3-azanyl-2-[3-[2-[2-[2-[2-[2-[2-[2-[2-[2-[2-[2-[2-[2-[2-[2-[2-[2-[[3-azanyl-1-[[2-[[3-methyl-6-[4-methyl-3-(methylsulfonyl-$l^{2}-azanyl)cyclohexa-1,3,5-trien-1-yl]-[1,2,4]triazolo[4,3-b]pyridazin-8-yl]-$l^{2}-azanyl]-2-oxidanylidene-ethyl]amino]-1-oxidanylidene-propan-2-yl]amino]-2-oxidanylidene-ethoxy]ethoxy]ethoxy]ethoxy]ethoxy]ethoxy]ethoxy]ethoxy]ethoxy]ethoxy]ethoxy]ethoxy]ethoxy]ethoxy]ethoxy]ethoxy]ethoxy]propanoylamino]-~{N}-[3-[[3-methyl-6-[4-methyl-3-(methylsulfonylamino)phenyl]-[1,2,4]triazolo[4,3-b]pyridazin-8-yl]amino]-3-oxidanylidene-propyl]propanamide 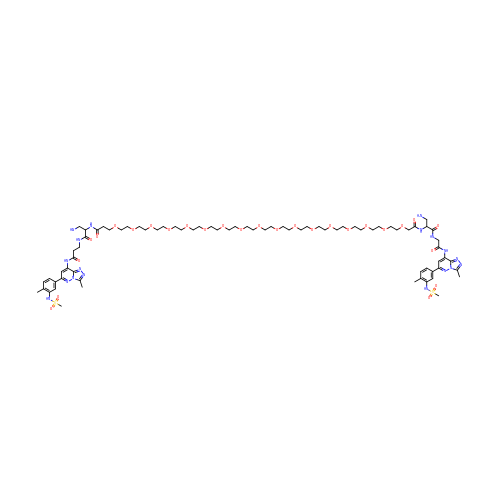| C76 H105 N18 O27 S2 | PSQFSMQXCFCIIU-UHFFFAOYSA-N>MALFGYARVSTSQQSLDIQVRALKDAGVKANRIFTDKASGSSSDRKGLDLLRMKVKEGDVILVKKLDRLGRDTADMIQLIKEFDAQGVSIRFIDDSIDTSSAMGRMVVTILSAVAQAERQRILQRTNEGRQEAMAKGVVFGRKRKIDRDAVLNMW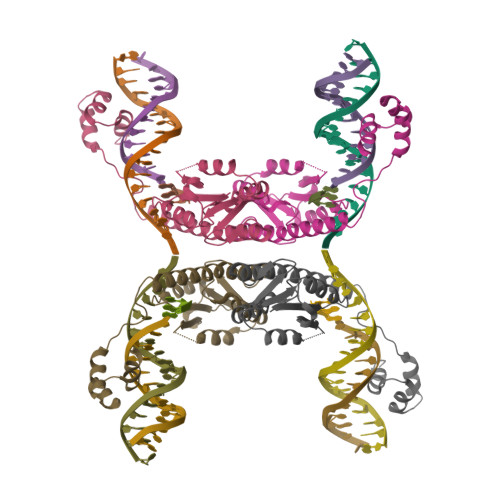QQGLGASHISKTMNIARSTVYKVINESN[2x]The norovirus genome contains three open reading frames (ORF1 to 3), where ORF1 encodes the nonstructural proteins, ORF2 encodes the capsid protein (VP1), and ORF3 encodes a minor structural protein (VP2). The S domain forms a scaffold surrounding the viral RNA, whereas the P domain contains the determinants of strain diversity and recognition of attachment factors. There is considerable antigenic drift among human noroviruses, and new genetic variants evolve every other year, which can result in new epidemics worldwide. It is well known that human noroviruses bind with various specificities to histo-blood group antigens (HBGAs), which are present in saliva, on the surface of epithelial cells, and in mucosal secretions. To elucidate the constraints on non-HBGA binders from a structural perspective, we determined the X-ray crystal structures of the capsid-protruding domains (P domains) of two GII.1 (HV and noro485) nonbinders and one GII.2 (SMV) HBGA nonbinder.

Similarly, a GII.2 strain, termed Snow Mountain virus (SMV), also failed to bind synthetic HBGAs but weakly bound HBGA B type in saliva. In contrast, SMV infections of human volunteers were shown to be independent of the blood type. HV, noro485, and SMV P domains diffracted to 1.86, 1.50, and 1.60 Å resolutions, respectively. Compared to the P domains of HV and noro485, that of SMV contained an insertion loop (SMV numbering; Ala345 to Ala351) in the P2 subdomain, which was also observed in a GII. In the HV and SMV P domains, we found two loop regions with disordered residues in the P2 subdomain, i.e., no discernible electron density, which suggested a certain degree of flexibility in these loops. In the HV P domain, Pro295 to Asp296 and Glu372 to Asp375 were disordered, while in the SMV P domain, residues Gln295 to Asp298 and Trp378 to Asp381 were disordered. The equivalent residues in the HV P domain were Cys345, Arg346, Asp375, and Gly438; in noro485, they were Cys345, Arg346, Asp375, and Gly438; and in SMV, they were Asn352, Arg353, Asp382, and Gly445. In the noro485 and SMV structures, Asp375 and Asp382, respectively, were pointing ~180° away from the fucose, whereas in the HV structure, Asp375 was missing because of the lack of electron density. In HV and SMV, loop B could not be modeled into the structures because of the lack of electron density. However, our new data indicate that Asp375 in HV, Asp375 in noro485, and Asp382 in SMV are unable to participate in the stabilization of the fucose moiety of HBGAs because of their flexibility or suboptimal orientation.

>GSKPFTLPILTLGELSNSRFPVSIDQMYTSPNEVISVQCQNGRCTLDGELQGTTQLQVSGICAFKGEVTAHLQDNGTLYNITITNLNGSPFDPSEDIPAPLGVPDFQGRVFGVITQRDKQNAAGQSQPANRGHDAVVPTYTAQYTPKLGQVQIGTWQTDDLKVNQPVKFTPVGLNDTEHFNQWVVPRYAGALNLNTNLAPSVAPVFPGERLLFFRSYLPLKGGYGNPAIDCLLPQEWVQHFYQEAAPSMSEVALVRYINPDTGRALFEAKLHRAGFMTVSSNTSAPVVVPANGYFRFDSWVNQFYSLAPM[3x]> SDAAPGASKLRAVLEKLKLSRDDISTAAGMVNG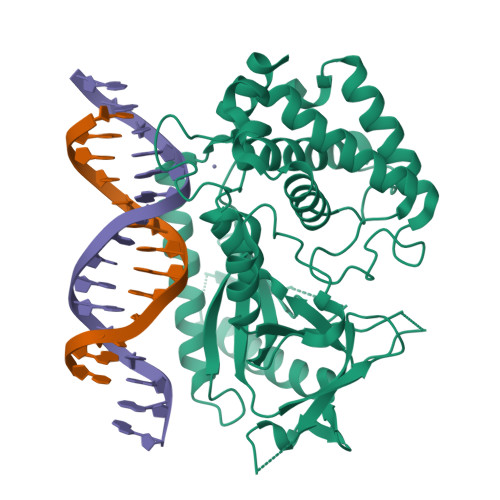VVDHLLRRLKCDSAFRGVGLLNTGSYYEHVKISAPNEFDVMFKLEVPRIQLEEYSNTRAYYFVKFKRNPKENPLSQFLEGEILSASKMLSKFRKIIKEEINDIKDTDVIMKRKRGGSPAVTLLISEKISVDITLALESKSSWPASTQEGLRIQNWLSAKVRKQLRLKPFYLVPKHAKEGNGFQEETWRLSFSHIEKEILNNHGKSKTCCENKEEKCCRKDCLKLMKYLLEQLKERFKDKKHLDKFSSYHVKTAFFHVCTQNPQDSQWDRKDLGLCFDNCVTYFLQCLRTEKLENYFIPEFNLFSSNLIDKRSKEFLTKQIEYERNNEFPVFDEF>[2x]SNAMSSVVVVGTQWGDEGKGKITDFLSEHAEVVARYQGGNNAGHTIVFGGVKYKLHLIPSGIFYKEKICVIGNGLVVDPKALLEELKYLHDRGVSTDNLRVSNRAHVILPYHLKQDELEEASKGDNKIGTTKKGIGPAYMDKAARIGIRMADLLD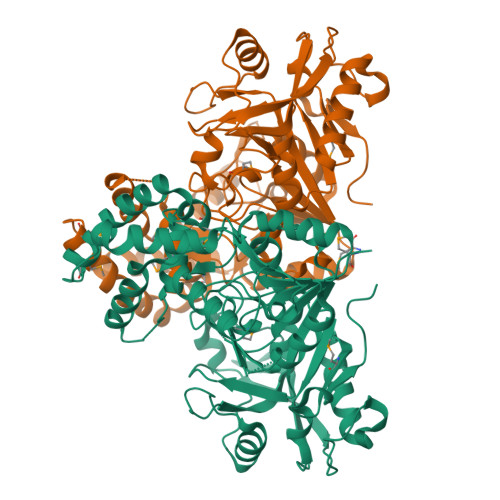REAFKEKLEQNLAQKNRLFEKMYDTEGFSVDEIFEEYFEYGQQIAQYVCDTSVVLNDALDNNHRVLFEGAQGVMLDIDHGTYPFVTSSNPIAGGVTVGTGVGPAKVTRVVGVCKAYTSRVGDGPFPTELHDEIGHQIREVGREYGTTTGRPRRVGWFDSVVVRHARRVSGLTDLSLNSIDVLTGIPTLKICVAYKCDGKVIDEVPANLNILAKCEPVCEELPGWTEDITGVRSLDELPENARKYVERVSELTGIQLSMFSVGPDRNQTNIVRNVYEA>GMSLAPWRGAIAHALHRNRSLVYARYLQLATVQPNGRPANRTLVFRGFLEDTNQLRFITDTRSAKADQIQQQPWAEICWYFPNTREQFRMAGDLTLISSDDSHQDLQPARIAMWQELSDAARLQFGWPYPGKPRIKESGAFEPSPPDPIEPVPNFCLLLLDPVQVDHLELRG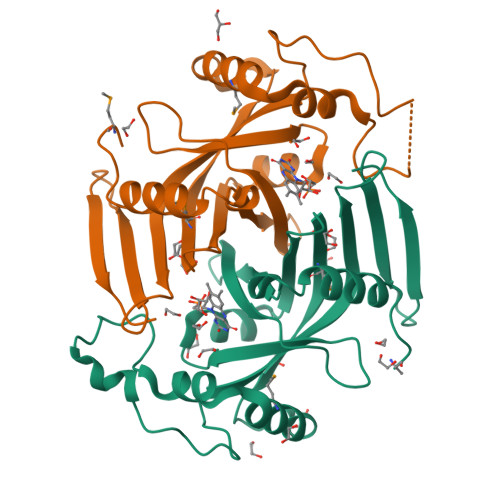EPQNRWLYHRNDQQEWSSEAINP[2x]6-FLUORO-2-(2'-FLUORO-1,1'-BIPHENYL-4-YL)-3-METHYLQUINOLINE-4-CARBOXYLIC ACID | C23 H15 F2 N 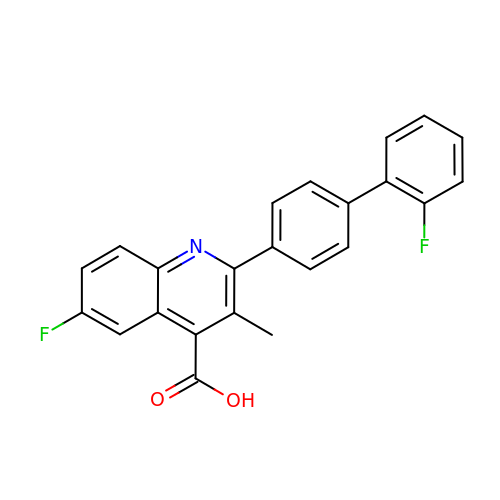O2 | PHEZJEYUWHETKO-UHFFFAOYSA-N>SSEQLQALLLEEVMNSSTLSQEVSDLVEMIWAEALGHLEHMLGSGSGSGGSKPNPPSLAKYRALRCKIEHVEQNTEEFLRVRKEVLQNHHSKSPVDVLQIFRVGRVNETTEFLSKLGNVRPLLHGSPVQNIVGILCRGLLLPKVVEDRGVQRTDVGNLGSGIYFSDSLSTSIKYSHPGETDGTRLLLICDVALGKCMDLHEKDFSLTEAPPGYDSVHGVSQTASVTTDFEDDEFVVYKTNQVKMKYIIKFSMPGDQIKD[3x]

PARP4 is an ADP-ribosyltransferase that resides within the vault ribonucleoprotein organelle. PARP4 is an ADP-ribosyltransferase that uses NAD+ as a substrate to synthesize ADP-ribose modifications on molecules. The PARP1-homology region of PARP4 includes a BRCT fold, a WGR domain, and the catalytic (CAT) domain. However, PARP3 and PARP4 contain the catalytic triad H-Y-E but are considered MARylation enzymes, indicating that other structural features are important determinants of catalytic output.

We also determined structures of the PARP4 ART domain alone (CATΔHD), which provided higher-resolution insights into the active site configuration that gives rise to PARP4 mono(ADP-ribosylation) activity. The HD was replaced with an 8-residue linker (GSGSGSGG) connecting L282 to S365. CATΔHD crystallized in complex with EB47, and in complex with NADH, the non-hydrolysable reduced form of NAD+. The CATΔHD/NADH crystals diffracted to 2.55 Å and belong to space group C2221 with three PARP4 molecules in the asymmetric unit. The structure was determined by molecular replacement using a truncated version of the PARP4 CAT/EB47 structure with the ligand removed. Two PARP4 molecules had NADH in their active sites, whereas the active site of the third molecule was empty due to a nearby crystal contact. The structure was refined to a crystallographic R/RFREE of 0.211/0.254. The structure of the PARP4 ART domain bound to NADH was compared to the closely related ART domains of PARP1, PARP2 and PARP3 in order to investigate the structural basis for the MARylation activity of PARP4. In the acceptor site, main chain atoms from residues L985 and Y986 in PARP1 interact with the α-phosphate of ADP, and the equivalent residues E544 and D545 of PARP4 are positioned such that they would clash with both the α- and β-phosphates. We thus conclude that PARP4 does not maintain a functional acceptor site as defined by the chicken PARP1 structure.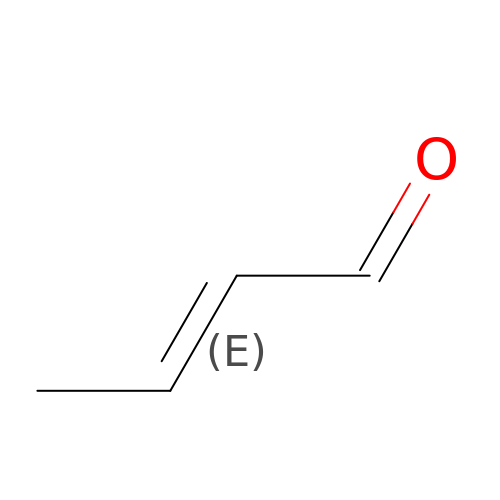(2E)-BUT-2-ENAL | C4 H6 O | MLUCVPSAIODCQM-NSCUHMNNSA-N>MASWSHPQFEKGASLDSPTFGCTDSPVRRERGQKAVFCGLTSIVWLHRKMQDAFFLVVGSRTCAHLLQAAAGVMIFAEPRFGTAVLEEQDLAGLADAHKELDREVAKLLERRPDIRQLFLVGSCPSEVLKLDLDRAAERLSGLHAPHVRVYSYTGSGLDTTFTQGEDTCLAAMVPTLDTTEAAELIVVGALPDVVEDQCLSLLTQLGVGPVRMLPARRSDIEPAVGPNTRFILAQPFLGETTGALERRGAKRIAAPFPFGEEGTTLWLKAVADAYGVSAEKFEAVTAAPRARAKKAIAAHLETLTGKSLFMFPDSQLEIPLARFLARECGMKTTEIATPFLHKAIMAPDLALLPSNTALTEGQDLEAQLDRHEAINPDLTVCGLGLANPLEAKGHATKWAIELVFTPVHFYEQAGDLAGLFSRPLRRRALLNGGAA[2x];>[2x]MKLTLWTYEGPPHVGAMRVATAMKDLQLVLHGPQGDTYADLLFTMIERRNARPPVSFSTFEASHMGTDTAILLKDALAAAHARYKPQAMAVALTCTAELLQDDPNGISRALNLPVPVVPLELPSYSRKENYGADETFRALVRALAVPMERTPEVTCNLLGATALGFRHRDDVAEVTKLLATMGIKVNVCAPLGASPDDLRKLGQAHFNVLMYPETGESAARHLERACKQPFTKIVPIGVGATRDFLAEVSKITGLPVVTDESTLRQPWWSASVDSTYLTGKRVFIFGDGTHVIAAARIAAKEVGFEVVGMGCYNREMARPLRTAAAEYGLEALITDDYLEVEKAIEAAAPELILGTQMERNIAKKLGLPCAVISAPVHVQDFPARYAPQM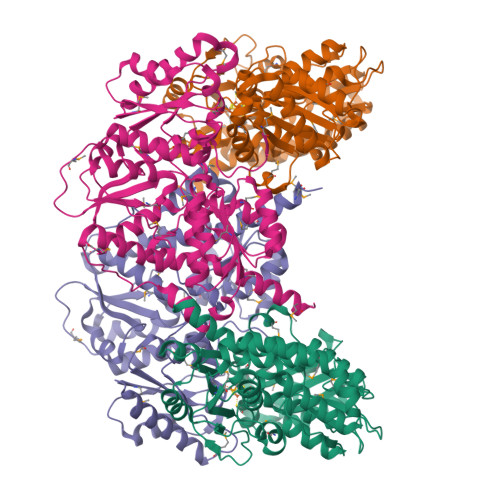GFEGANVLFDTWVHPLVMGLEEHLLTMFREDFEFHDAAGASHHGGKAVAREESPVAPADLAPAATSDTPAAPSPVVVTQASGEIRWMPEAERELRKIPFFVRGKAKRNTELYAAHKGVCDITVETLYEAKAHYAR>XGELAQALKELAKALKE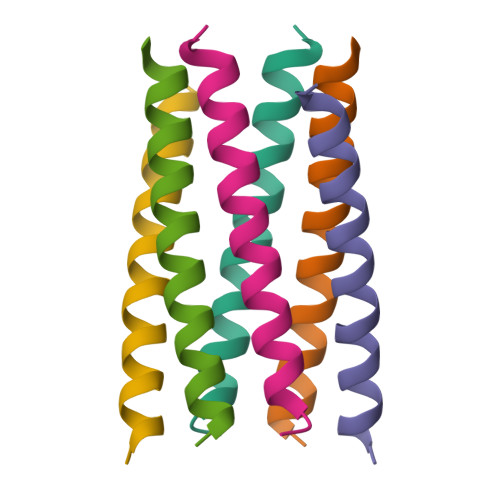LAWALKELAQALKGX[3x]>[2x]GHMRIGIISVGPGNIMNLYRGVKRASENFEDVSIELVESPRNDLYDLLFIPGVGHFGEGMRRLRENDLIDFVRKHVEDERYVVGVCLGMQLLFEESEEAPGVKGLSLIEGNVVKLRSRRLP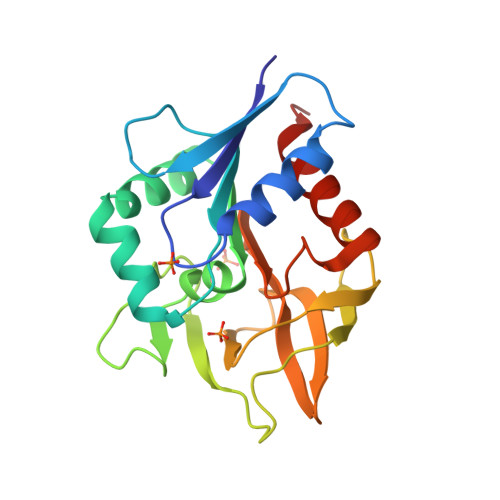HMGWNEVIFKDTFPNGYYYFVHTYRAVCEEEHVLGTTEYDGEIFPSAVRKGRILGFQFHPEKSSKIGRKLLEKVIECSLSRRGS Quinolinate phosphoribosyltransferase (QAPRTase) is an essential enzyme in the first step of NAD+ biosynthesis, catalyzing the transfer of the phosphoribosyl moiety from PRPP to QUIN to generate NAMN. NAD+ biosynthesis is essential for all organisms. In de novo NAD+ biosynthesis, the two precursors quinolinate (QUIN) and nicotinate receive a phosphoribosyl moiety from 5-phosphoribosyl-1-pyrophosphate (PRPP) via the respective phosphoribosyltransferases. QAPRTase is reported to exist as a dimer or a hexamer depending on the source.

In Homo sapiens, Rattus norvegicus, and Sus scrofa, QAPRTases were reported to exist as hexamers. Although several QAPRTase structures have been determined as a result of extensive crystallographic studies, structural information regarding the reaction mechanism of QAPRTase in higher eukaryotes, including mammals, is limited due to the lack of a structure in complex with a reactant or product. Here, we report the 2.1 Å resolution crystal structure of Sus scrofa QAPRTase (Ss-QAPRTase) in complex with NAMN. Our results represent the first crystal structure of a mammalian hexameric QAPRTase with its reaction product and may provide structural information useful for understanding the mode of binding of NAMN with eukaryotic QAPRTases and for designing drugs specifically targeting the QAPRTases of pathogenic bacteria rather than those of mammals.

>MDPEGLALLLPPATLATLADSWLREDCPGLNPVALVTGAAPSQAVLWAKSPGILAGRPFFDAIFAQVNCQVSWFLPEGSKLVPVAKVAEVRGPAHCLLLGERVALNMLARCSGVASAAATAVETARGTGWAGHVAGTRKTTPGFRLVEKYGLLVGGATSHRYDLGGLVMVKDNHVVAAGGVKQAVQGARRAANFALKVEVECSSLQEALEAAEAGADLVLLDNFRPEELHPTAAALKAQFPTVGVEASGGVTLDNLPQFCGPHIDVISLGMLTQAAPALDFSLKLFAE[2x]> GDSLSIHQLAAQGELDQLKEHLRKGDNLVN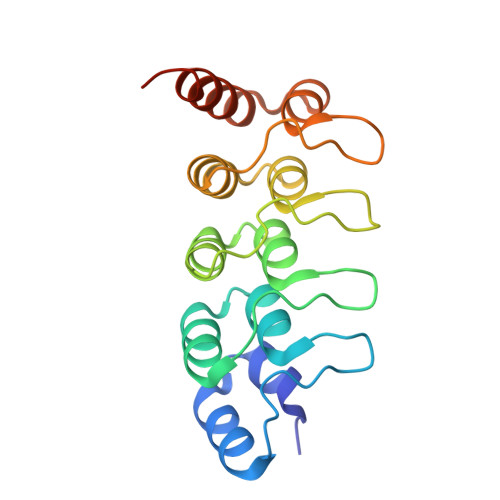KPDERGFTPLIWASAFGEIETVRFLLEWGADPHILAKERESALSLASTGGYTDIVGLLLERDVDINIYDWNGGTPLLYAVRGNHVKCVEALLARGADLTTEADSGYTPMDLAVALGYRKVQQVIENHILKLFQSNLVPADPE>[4x]MHHHHHHTSKIEQPRWASKDSAAGAASTPDEKIVLEFMDALTSNDAAKLIEYFAEDTMFQAMPLPPAYGRDAVEQTLAGLFTVMSFDAVETFHIGSSNGLVYTERVDVLRALPTGKSYNVSVLGVFQLTEGKITGWRDYFDLREFEEAVDLPLRG

We report an in silico strategy for the biocatalytic synthesis of chiral N- and O-heterocycles via Baldwin cyclization modes of hydroxy- and amino-substituted epoxides and oxetanes using the limonene epoxide hydrolase from Rhodococcus erythropolis. We turned to cofactor-independent limonene epoxide hydrolases (LEHs) that normally catalyze direct hydrolysis of epoxides by positioning and activating water at the active site. On the basis of the well-documented mechanism of ReLEH, a water molecular is positioned by H-bonds to N55 and Y53 while D132 abstracts a proton from the water, enabling a smooth nucleophilic attack on one of the substrate’s epoxide carbon center. We have rationally engineered the epoxide hydrolase ReLEH with construction of a general platform for Baldwin cyclization reactivity of hydroxy- and amino-epoxides and oxetanes.

In curiosity-driven experiments, the mutants SZ612 (Y53F/N55A/I80F/L114V/I116V) and SZ621 (Y53F/N55A/I80F/I116V) produced only the Baldwin product 2 with none of 3 nor of the vicinal diol 4 as side-products. In order to gain insights on the active substrate-LEH interactions, the X-ray structures of the key variants SZ612 and SZ616 were analyzed. Consequently, the representative substrates in complex with LEH mutants, including the models SZ612‒(R)-1 and SZ616‒(R)-1, were constructed by molecular docking. Following the docking analysis, the epoxy ring O-atom of the substrate consistently establishes a hydrogen-bond interaction with the protonated catalytically active D101; the aforementioned hydrogen-bond network with water molecular is terminated by substitutions Y53F and N55A, enabling the substrate distal hydroxyl moiety to form a hydrogen-bond interaction with the deprotonated D132. In model SZ612‒(R)-1, the dihedral angle θ was mainly gathered between 0o and 180o during the MD simulations, suggesting that attack from the Re-face is unsupportive for SZ612. Moreover, for both of the SZ612 and SZ616 mutants, the slightly shorter distance d1 was observed during the simulations, indicating that the ON atom preferentially attacks C1. Furthermore, to better illustrate the bond forming and breaking in the Baldwin/anti-Baldwin selection pathways, the hybrid QM/MM scheme was employed, enabling the calculation the activation energy barriers. It is of interest to note that the shorter distance d2 allows a relatively low activation energy, and hence the formation of Baldwin product is favored for the two variants.> MLQFYRNLGKSGLRVSCLGLGTWVTFGGQITDEMAEHLMTLAYDNGINLFDTAEVYAAGKAEVVLGNIIKKKGWRRSSLVITTKIFWGGKAETERGLSRKHIIEGLKASLERLQLEYVDVVFANRPDPNTPMEETVRAMTHVINQGMAMYWGTSRWSSMEIMEAYSVARQFNLIPPRCEQAEYHMFQREKVEVQLPELFHKIGVGAMTWSPLACGIVSGKYDSGIPPY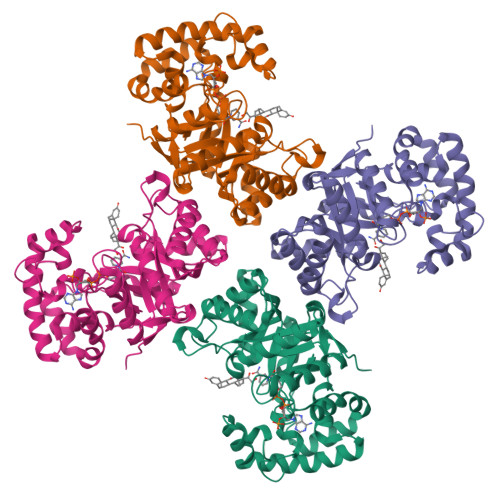SRASLKGYQWLKDKILSEEGRRQQAKLKELQAIAERLGCTLPQLAIAWCLRNEGVSSVLLGASNAEQLMENIGAIQVLPKLSSSIVHEIDSILGNKPYS> HHHHHHGGCPSQCSCRGTYVDCDSRRLASVPAGIPTNVQILNLYNNQITNLEPGVFDRL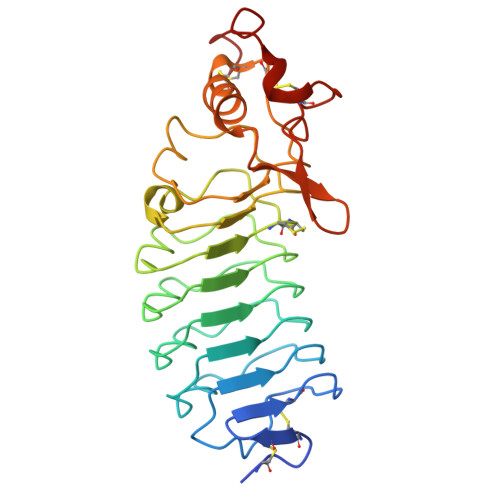VNLQKLYLSGNQLQALPVGVFDKLSQLTFLSLDENKLTALPNGVFDKLTELTYLNLNTNQLTALPEGVFDRLVHLKELLMCCNKLTELPRGIERLTHLTHLALDQNQLKSIPHGAFDRLSSLTHAYLFGNPWDCECRDIMYLRNWVADHTSIVMRWDGKAVNDPDSAKCAGTNTPVRAVTEASTSPSKC N-2-(biphenyl-4-ylsulfonyl)-N-2-(isopropyloxy)-acetohydroxamic 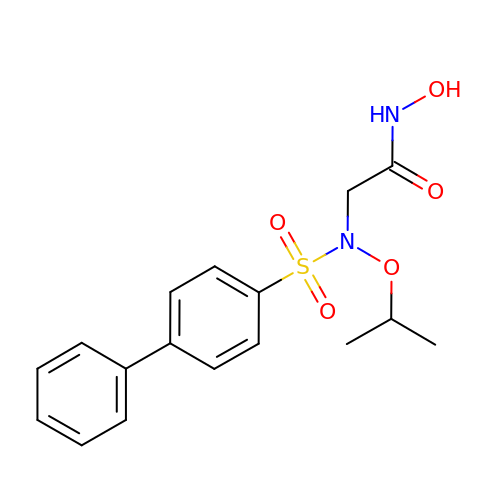acid | C17 H20 N2 O5 S | PHGLPDURIUEELR-UHFFFAOYSA-N> GMPHVHVSTDNSLLDIGLIHRTLSQDTDWAKDIPLALVQRAIDHSLCFGGFVDGRQVAFARVISDYATFAYLGDVFVLPEHRGRGYSKALMDAVMAHPDLQGLRRFSLATSDAHGLYARYGFTPPLFPQS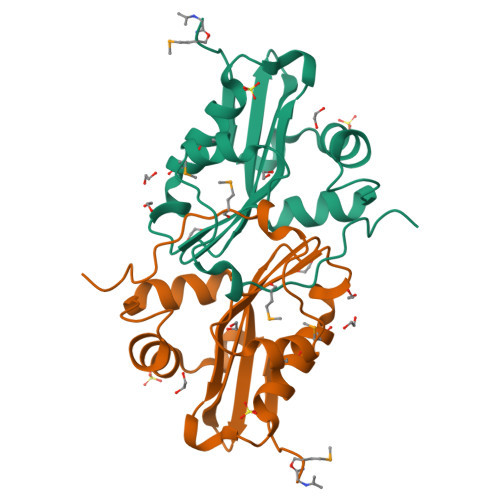LMERYVPGLYST> MAPARPNWLAYDWGLVFLVAAIVALGFVNLGSAAPDPVLLYRQSVALGLGLLLAFLLQFLSRRRLFGLAYPLYGASLLLLALVLVVGREINGARAWFVLGPLQFQPLELAKLGLLLALAKALEGRPIARVWDYALPALLTLPVVGLLLLQPDLGGALVVLFGVFVVVFVRGLPWRHLLVGLFALALLVPTAVWPNLKPYQRERVLIVLDPYRDPLGQGFQVIQSTIAIGSGGLFGKGYGQGTQAQLGFIPFRHTAFVFSVWAEEWGFVGVVGLLGLYGLLLAR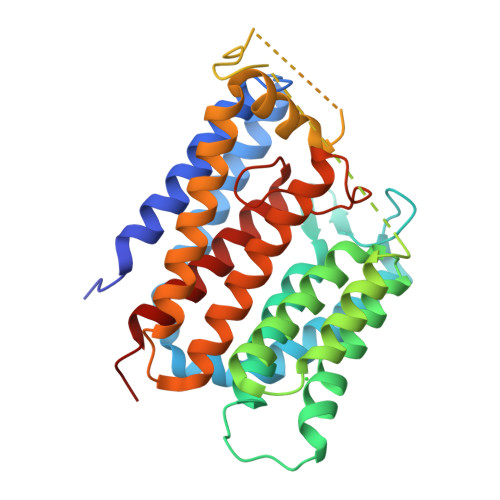LFALALACPRLSDRLFLSGFAGMLGFQVVVNLGVALGVMPVTGLTLPLFSYGGSSLIATLAGLGLVLLVHRDRYQD Angiogenin (ANG), a 14-kDa basic protein is an angiogenic ribonuclease and member of the bovine pancreatic ribonuclease (RNase A) family (also known as RNase 5). Like RNase A, ANG cleaves preferentially on the 3′ side of pyrimidines and follows a transphosphorylation/hydrolysis mechanism. In addition, the crystal structure of human ANG has revealed that it has an RNase A fold and the catalytic triad (residues H13, K40 and H114) is conserved. The enzymatic activity of ANG is several orders of magnitude lower than that of RNase A towards conventional RNase substrates, but essential for its angiogenic effect.

In the native ANG structure F100 and V103 residues (located on β5 and β6 strands respectively) are in close proximity to the substrate binding site involving residue E108. The results from two variant structures F100I and V103I are analyzed here and both the variant residues are well defined in their respective electron density maps. On the other hand, in the V103I ALS variant structure, the side chain seems to have gained additional interactions with residues I46, I56 and F76 making the hydrophobic core more stable. This provides some structural explanation for the altered catalytic activity for this variant.

> MQDNSRYTHFLTQHYDAKPQGRDDRYCESIMRRRGLTSPCKDINTFIHGNKRSIKAICENKNGNPHRENLRISKSSFQVTTCKLHGGSPWPPCQYRATAGFRNIVVACENGLPVHLDQSIFRRP>MGSETPQAEVGPTGCPHRSGPHSAKGSLEKGSPEDKEAKEPLWIRPDAPSRCTWQLGRPASESPHHHTAPAKSPKILPDILKKIGDTPMVRINKIGKKFGLKCELLAKCEFFNAGGSVKDRISLRMIEDAERDGTLKPGDTIIEPTSGNTGIGLALAAAVRGYRCIIVMPEKMSSEKVDVLRALGAEIVRTPTNARFDSPSSHVGVAWRLKNEIPNSHILDQYRNASNPLAHYDTTADEILQQCDGKLDMLVASVGTGGTITGIARKLKEKCPGCRIIGVDPEGSILAEPEELNQTEQTTYEVEGIGYDFIPTVLDRTVVDKWFKSNDEEAFTFARMLIAQEGLLCGGSAGSTVAVAVKAAQELQEGQRCVVILPDSVRNYMTKFLSDRWMLQKGFLKEEDLTEKKPWWWHLR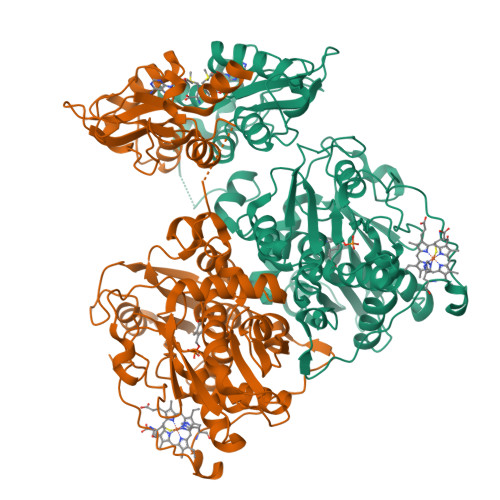VQELGLSAPLTVLPTITCGHTIEILREKGFDQAPVVDEAGVILGMVTLGNMLSSLLAGKVQPSDQVGKVIYKQFKQIRLTDTLGRLSHILEMDHFALVVHEQQRQMVFGVVTAIDLLNFVAAQERDQKELHHHHHH[2x]> MGSSHHHHHHSSGLVPRGSMAEKFESRGIEEASSEVPTQRRCGAMEVHHRLLRSASYVRERDQIENLALKYKQGFRAISRMEIVKIPVVVHVVWNEEEENISDAQIQSQIDILNKDFRKLNSDVSQVPSVWSNLIADLGIEFFLATKDPNGNQTTGITRTQTSVTFFTTSDEVKFASSGGEDAWPADRYLNIWVCHVLKSEIGQDILGYAQFPGGPAETDGVVIVDAAFGTTGTALPPFDKGRTATHE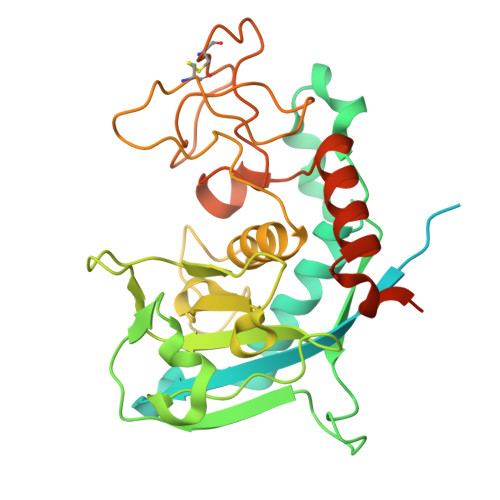IGHWLNLYHIWGDELRFEDPCSRSDEVDDTPNQADPNFGAPSYPHVSCSNGPNGDMFMNYMDYVDDKCMVMFTQGQATRVNACLDGPRSSFLARVEETEKKEAPSKREMPMPR methyl 4-propanoyl-1~{H}-pyrrole-2-carboxylate | C9 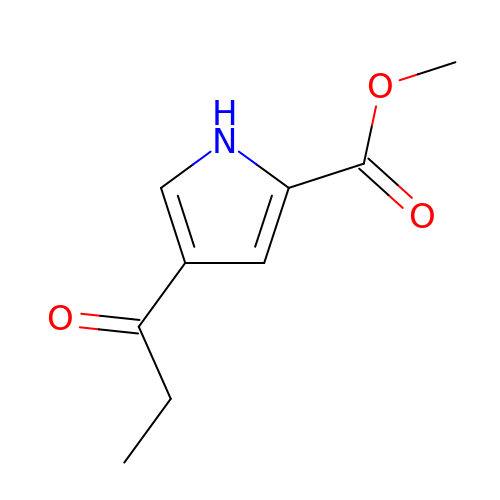H11 N O3 | GMDIDIYLWBUNEW-UHFFFAOYSA-N> MNHKVHHHHHHMVTVVYQNGLPVISVRLPSRRERCQFTLKPISDSVGVFLRQLQEED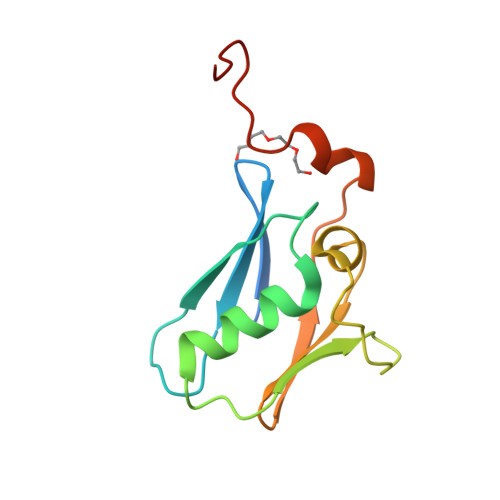RGIDRVAIYSPDGVRVAASTGIDLLLLDDFKLVINDLTYHVRPPKRDLLSHENAATLNDVKTLVQQ>[2x]MTDVNASSESRLAA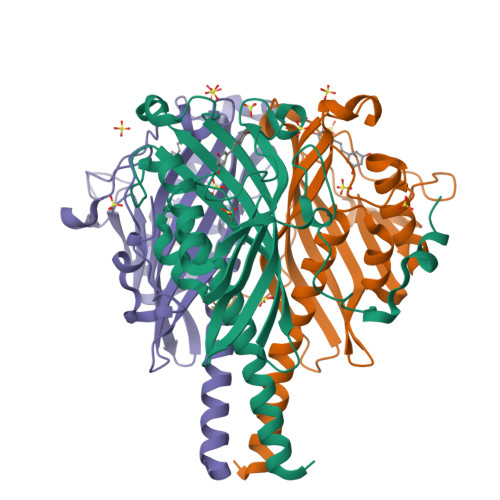LEARVTELEDLNAIRRLQWAYGYYIDYNRPEEVAGLFAKDGAVVFLSGEYVGYEGVMRLYGTWFQNLFTGGRRGPVHGLLLDHFQLQDVITIAPDGQTAKGRFRGILAGGWHDDIVKDKPEGMPQQFWESGIYENDYVKEDGVWKIKRLDYMMQWQADYETGWSKTIAHLQPAAVCFPENPIGPDRLLPETEVRQTWPHRAEVPMSFAHPVLAKAFAVGEFTKLQKKWPLEHHHHHH>MPEKSLYEMAVEQFNRAASLMDLESDLAEVLRRPKRVLIVEFPVRMDDGHVEVFTGYRVQHNVARGPAKGGIRYHPDVTLDEVKALAFWMTWKTAVMNLPFGGGKGGVRVDPKKLSRNELERLSRRFFSEIQVIIGPYNDIPAPDVNTNADVIAWYMDTYSMNVGHTVLGIVTGKPVELGGSKGREEATGRGVKVCAGLAMDVLGIDPKKATVAVQGFGNVGQFAALLISQELGSKVVAVSDSRGGIYNPEGFDVEELIRYKKEHGTVVTYPKGERITNEELLELDVDILVPAALEGAIHAGNAERIKAKAVVEGANGPTTPEADEILSRRGILVVPDILANAGGVTVSYFEWVQDLQSFFWDLDQ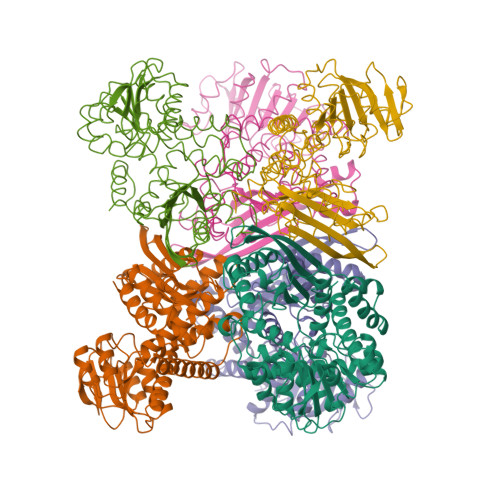VRNALEKMMKGAFNDVMKVKEKYNVDMRTAAYILAIDRVAYATKKRGIYP[6x]>[2x]MVKQIESKTAFQEALDAAGDKLVVVD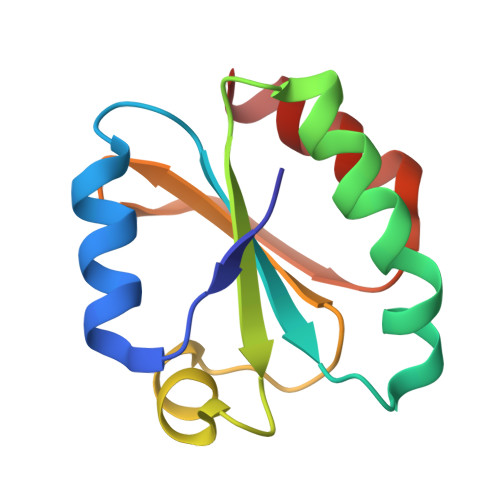FSATWCGPCKMIKPFFHSLSEKYSNVIFLEVDVDDCQDVASESEVKSMPTFQFFKKGQKVGEFSGANKEKLEATINELV>MSQEALKAPVVVLGAGLASVSFVAE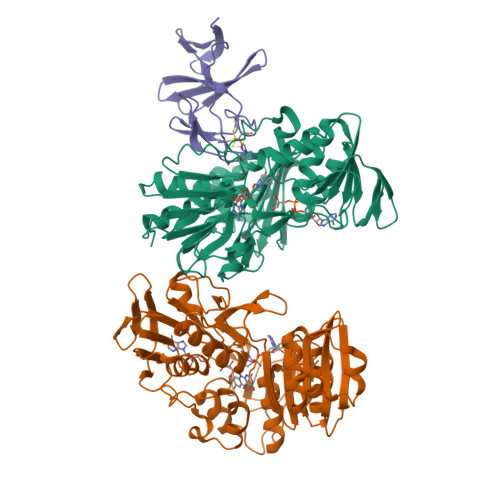LRQAGYQGLITVVGDEAERPYDRPPLSKDFMAHGDAEKIRLDCKRAPEVEWLLGVTAQSFDPQAHTVALSDGRTLPYGTLVLATGAAPRALPTLQGATMPVHTLRTLEDARRIQAGLRPQSRLLIVGGGVIGLELAATARTAGVHVSLVETQPRLMSRAAPATLADFVARYHAAQGVDLRFERSVTGSVDGVVLLDDGTRIAADMVVVGIGVLANDALARAAGLACDDGIFVDAYGRTTCPDVYALGDVTRQRNPLSGRFERIETWSNAQNQGIAVARHLVDPTAPGYAELPWYWSDQGALRIQVAGLASGDEEIVRGEVSLDAPKFTLIELQKGRIVGATCVNNARDFAPLRRLLAVGAKPDRAALADPATDLRKLAAAVAA[2x];> MTFTKACSVDEVPPGEALQVSHDAQKVAIFNVDGEFFATQDQCTHGEWSLSEGGYLDGDVVECSLHMGKFCVRTGKVKSPPPCEPLKVYPIRIEGRDVLVDFSRAALHA> PSANDGPSFTTSKTSQNTTSENVHFVDGDTPWTYDVAATPDETSKLSGFD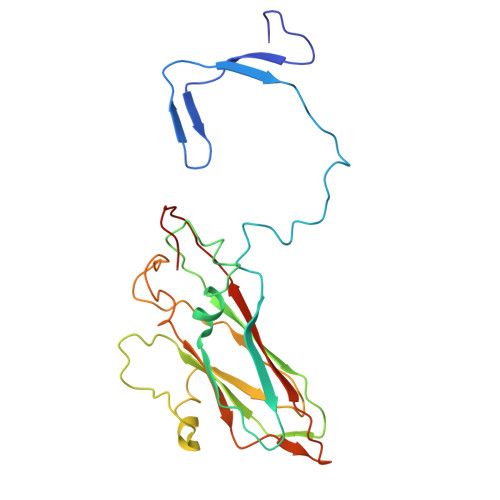DAGLGEFLSRPIKIQQYQWTPGVQLFQTFNPWSDYFGNADVLEKINRFRNLRCKLCLKVLINGNSFYYGRALLSYNPYLRNDQVTVNRSFFIQDLIAASNKPHILLDPCSSEGGQMCLPFIWPENYLDITSTGWEDQMGECIIHDFDVLRHANGGTDPITVSIFAWAEDVSLLIPTTVAAQ Glycoprotein 130 (gp130) is a signaling receptor shared by interleukin-6 (IL-6) family cytokines (or gp130 family cytokines), including IL-6, ciliary neurotrophic factor (CNTF), cardiotrophin-like cytokine factor 1 (CLCF1), leukemia inhibitory factor (LIF), oncostatin M (OSM), cardiotrophin-1 (CT-1), IL-11, IL-27, IL-35, and IL-39 (1). These cytokines share a canonical four-helix bundle structure in which four major helices (termed helices A to D) are linked by three loops (termed AB, BC, and CD loops), as well as three conserved receptor binding epitopes (termed sites 1 to 3). IL-6 and IL-11 signal through gp130 homodimerization, while other cytokines require another “tall” signaling receptor, such as LIF receptor (LIFR) or IL-27 receptor subunit alpha (IL-27Rα), which forms a heterodimer with gp130 for signal transduction. The extracellular domains (ECDs) of gp130 include an N-terminal immunoglobulin (Ig)–like domain (D1), a cytokine-binding homology region (CHR, D2D3), and three membrane-proximal fibronectin type III domains (FNIII, D4 to D6).

CLCF1 was also found to interact with CNTFRα and signal via the gp130-LIFR heterodimer analogous to CNTF, and cytokine receptor–like factor 1 (CRLF1) was shown to chaperone the secretion of CLCF1 (6). The bottom centers of LIFR and gp130 juxtamembrane domains are positioned ~22 Å apart, comparable to that seen in the CNTF complex. CNTFRαF172 also serves as the anchor point of the CNTFRα-CLCF1 interface by engaging T193, W196, R197, and K200 of CLCF1. Multiple electrostatic interactions are observed between positively charged CLCF1 residues (R48, R95, and K200) and negatively charged CNTFRα residues (D234, D284, and E286). Key gp130 residues engaging CNTF maintain their roles in the CLCF1 complex, with F191 engaging K42, D45, L46, and Y49 of CLCF1 helix A; D215 forming a hydrogen bond with CLCF1K42 at the center of the interface; and W164 capturing the middle portion of CLCF1 helix C. Similarly, site 2b (1325 Å2) has a larger buried surface area than site 2a (944 Å2) in the CLCF1 complex and greatly increases interactions at the composite site 2, which may explain why CNTFRα is indispensable for CLCF1 signaling. Like F152 and K155 of CNTF, the two conserved CLCF1 residues F178 and K181 also serve as key anchor points engaging LIFR residues (S310, N313, V315, I322, G324, and V326), consistent with previous mutagenesis studies. Notably, 72% of CLCF1 residues contributing to the packing of this interface are nonpolar, which is much higher than the percentage of nonpolar CNTF residues at the CNTF-LIFR interface (44%). We found that the CLCF1 complex and IL-27 complex appear to be more unstable than the other signaling complexes we characterized since the particles imaged in the cryo-EM experiments for both samples showed a very low percentage of full complex (~2%).

> ELLDPCGYISPESPVVQLHSNFTAVCVLKEKCMDYFHVNANYIVWKTNHFTIPKEQYTIINRTASSVTFTDIASLNIQLTCNILTFGQLEQNVYGITIISGLPPEKPKNLSCIVNEGKKMRCEWDGGRETHLETNFTLKSEWATHKFADCKAKRDTPTSCTVDYSTVYFVNIEVWVEAENALGKVTSDHINFDPVYKVKPNPPHNLSVINSEELSSILKLTWTNPSIKSVIILKYNIQYRTKDASTWSQIPPEDTASTRSSFTVQDLKPFTEYVFRIRCMKEDGKGYWSDWSEEASGITYEDRPSKAPSFWYKIDPSHTQGYRTVQLVWKTLPPFEANGKILDYEVTLTRWKSHLQNYTVNATKLTVNLTNDRYLATLTVRNLVGKSDAAVLTIPACDFQATHPVMDLKAFPKDNMLWVEWTTPRESVKKYILEWCVLSDKAPCITDWQQEDGTVHRTYLRGNLAESKCYLITVTPVYADGPGSPESIKAYLKQAPPSKGPTVRTKKVGKNEAVLEWDQLPVDVQNGFIRNYTIFYRTIIGNETAVNVDSSHTEYTLSSLTSDTLYMVRMAAYTDEGGKDGPEFTFTTPKFAQGEIEEQKLISEEDLGGEQKLISEEDLHHHHHH;> QKKGAPHDLKCVTNNLQVWNCSWKAPSGTGRGTDYEVCIENRSRSCYQLEKTSIKIPALSHGDYEITINSLHDFGSSTSKFTLNEQNVSLIPDTPEILNLSADFSTSTLYLKWNDRGSVFPHRSNVIWEIKVLRKESMELVKLVTHNTTLNGKDTLHHWSWASDMPLECAIHFVEIRCYIDNLHFSGLEEWSDWSPVKNISWIPDSQTKVFPQDKVILVGSDITFCCVSQEKVLSALIGHTNCPLIHLDGENVAIKIRNISVSASSGTNVVFTTEDNIFGTVIFAGYPPDTPQQLNCETHDLKEIICSWNPGRVTALVGPRATSYTLVESFSGKYVRLKRAEAPTNESYQLLFQMLPNQEIYNFTLNAHNPLGRSQSTILVNITEKVYPHTPTSFKVKDINSTAVKLSWHLPGNFAKINFLCEIEIKKSNSVQEQRNVTIKGVENSSYLVALDKLNPYTLYTFRIRCSTETFWKWSKWSNKKQHLTTEASPSKGPDTWREWSSDGKNLIIYWKPLPINEANGKILSYNVSCSSDEETQSLSEIPDPQHKAEIRLDKNDYIISVVAKNSVGSSPPSKIASMEIPNDDLKIEQVVGMGKGILLTWHYDPNMTCDYVIKWCNSSRSEPCLMDWRKVPSNSTETVIESDEFRPGIRYNFFLYGCRNQGYQLLRSMIGYIEELAPIVAPNFTVEDTSADSILVKWEDIPVEELRGFLRGYLFYFGKGERDTSKMRVLESGRSDIKVKNITDISQKTLRIADLQGKTSYHLVLRAYTDGGVGPEKSMYVVTKENSEQKLISEEDLGGEQKLISEEDLHHHHHH;> QRHSPQEAPHVQYERLGSDVTLPCGTANWDAAVTWRVNGTDLAPDLLNGSQLVLHGLELGHSGLYACFHRDSWHLRHQVLLHVGLPPREPVLSCRSNTYPKGFYCSWHLPTPTYIPNTFNVTVLHGSKIMVCEKDPALKNRCHIRYMHLFSTIKYKVSISVSNALGHNATAITFDEFTIVKPDPPENVVARPVPSNPRRLEVTWQTPSTWPDPESFPLKFFLRYRPLILDQWQHVELSDGTAHTITDAYAGKEYIIQVAAKDNEIGTWSDWSVAAHATPWTEEPRHLTTEAQAAETTTSTTSSLAPPPTTKICDPGELGSGGGP;> LNRTGDPGPGPSIQKTYDLTRYLEHQLRSLAGTYLNYLGPPFNEPDFNPPRLGAETLPRATVDLEVWRSLNDKLRLTQNYEAYSHLLCYLRGLNRQAATAELRRSLAHFCTSLQGLLGSIAGVMAALGYPLPQPLPGTEPTWTPGPAHSDFLQKMDDFWLLKELQTWLWRSAKDFNRLKKKMQPPAAAVTLHLGAHGFHHHHHH>[4x]MAHCTEYMNAPKKLPADVAEELATTAQKLVQAGKGILAADESTQTIKKRFDNIKLENTIENRASYRDLLFGTKGLGKFISGAILFEETLFQKNEAGVPMVNLLHNENIIPGIKVDKGLVNIPCTDEEKSTQGLDGLAERCKEYYKAGARFAKWRTVLVIDTAKGKPTDLSIHETAWGLARYASICQQNRLVPIVEPEILADGPH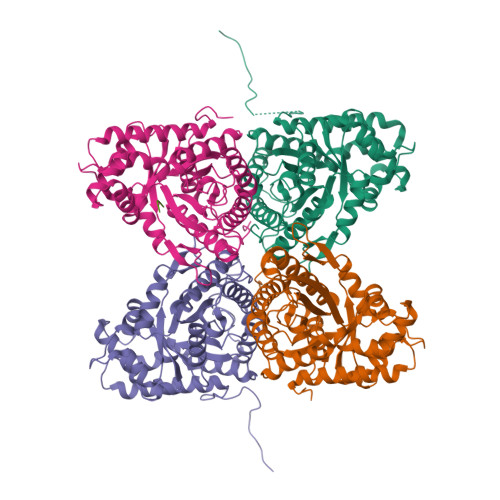SIEVCAVVTQKVLSCVFKALQENGVLLEGALLKPNMVTAGYECTAKTTTQDVGFLTVRTLRRTVPPALPGVVFLSGGQSEEEASVNLNSINALGPHPWALTFSYGRALQASVLNTWQGKKENVAKAREVLLQRAEANSLATYGKYKGGAGGENAGASLYEKKYVY;> EDNDWN>ATTYNAVVSKSSSDGKTFKTIADAIASAPAGSTPFVILIKNGVYNERLTITRNNLHLKGESRNGAVIAAATAAGTLKSDGSKWGTAGSSTITISAKDFSAQSLTIRNDFDFPANQAKSDSDSSKIKDT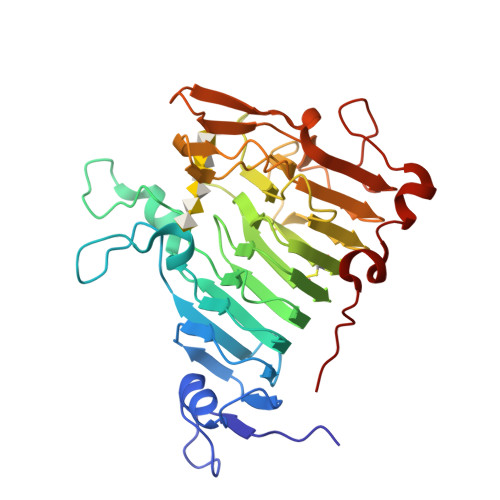QAVALYVTKSGDRAYFKDVSLVGYQDTLYVSGGRSFFSDCRISGTVDFIFGDGTALFNNCDLVSRYRADVKSGNVSGYLTAPSTNINQKYGLVITNSRVIRESDSVPAKSYGLGRPWHPTTTFSDGRYADPNAIGQTVFLNTSMDNHIYGWDKMSGKDKNGNTIWFNPEDSRFFEYKSYGAGATVSKDRRQLTDAQAAEYTQSKVLGDWTPTLP[2x]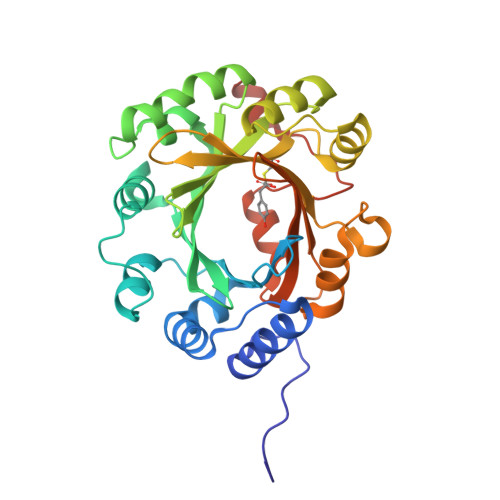> GSHMPALPIDQEFDCERFRADIRATAAAIGAPIAHRLTDTVLEAFRDNFAQGATLWKTTSQPGDQLSYRFFSRLKMDTVSRAIDAGLLDAAHPTLAVVDAWSSLYGGAPVQSGDFDAGRGMAKTWLYFGGLRPAEDILTVPALPASVQARLKDFLALGLAHVRFAAVDWRHHSANVYFRGKGPLDTVQFARIHALSGSTPPAAHVVEEVLAYMPEDYCVAITLDLHSGDIERVCFYALKVPKNALPRIPTRIARFLEVAPSHDVEECNVIGWSFGRSGDYVKAERSYTGNMAEILAGWNCFFHGEEGRDHDLRALHQHTESTMGGAR>[2x]MNAQAEEFKKYL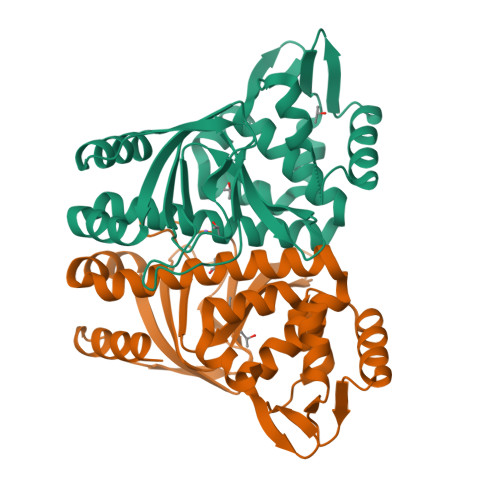ETNGIKPKQFHKKELIFNQWDPQEYCIFLYDGITKLTSISENGTIMNLQYYKGAFVIMSGFIDTETSVGYYNLEVISEQATVYVIKINELKELLSKNLTHFFYVFQTLQKQVSYSLAKFNDFSINGKLGSICGQLLILTYVYGKETPDGIKITLDNLTMQELGYSSGIAHSSAVSRIISKLKQEKVIVYKNSCFYVQNLDYLKRYAPKLDEWFYLACPATWGKLN> MSADSSPLVGSTPTGYGTLTIGTSIDPLSSSVSSVRLSGYCGSPWRVIGYHVVVWMMAGIPLLLFRWKPLWGVRLRLRPCNLAHAETLVIEIRDKEDSSWQLFTVQVQTEAIGEGSLEPSPQSQAEDGRSQAAVGAVPEGAWKDTALHKSEEAVSVGQKRVLRYYLFQGQRYIWIETQQAFYQVSLLDHGRSCDDVHRSRHGLSLQDQMVRKAIYGPNVISIPVKSYPQLLVDEALNPYYGFQAFSIALWLADHYYWYALCIFLISSISICLSLYKTRKQSQTLRDMVKLSMRVCVCRPGGEEEWVDSSELVPGDCLVLPQEGGLMPCDAALVAGECMVNESSLTGESIPVLKTALPEGLGPYCAETHRRHTLFCGTLILQARAYVGPHVLAVVTRTGFCTAKGGLVSSILHPRPINFKFYKHSMKFVAALSVLALLGTIYSIFILYRNRVPLNEIVIRALDLVTVVVPPALPAAMTVCTLYAQSRLRRQGIFCIHPLRINLGGKLQLVCFDKTGTLTEDGLDVMGVVPLKGQAFLPLVPEPRRLPVGPLLRALATCHALSRLQDTPVGDPMDLKMVESTGPQLQAMEEPPVPVSVLHRFPFSSALQRMSVVVAWPGATQPEAYVKGSPELVAGLCNPETVPTDFAQMLQSYTAAGYRVVALASKPLPTVPSLEAAQQLTRDTVEGDLSLLGLLVMRNLLKPQTTPVIQALRRTRIRAVMVTGDNLQTAVTVARGCGMVAPQEHLIIVHATGQPASLEFLPMESPTAVNGVKDPDQAASYTVEPDPRSRHLALSGPTFGIIVKHFPKLLPKVLVQGTVFARMAPE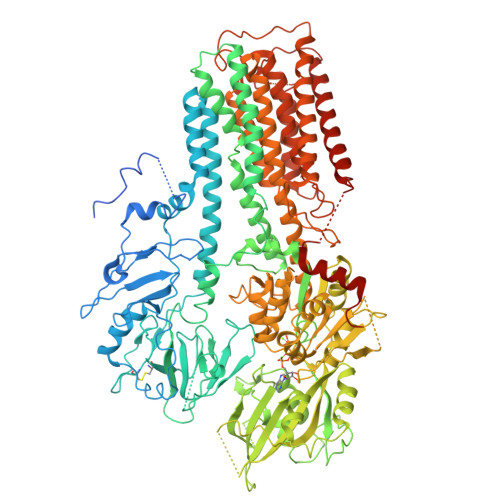QKTELVCELQKLQYCVGMCGDGANDCGALKAADVGISLSQAEASVVSPFTSSMASIECVPMVIREGRCSLDTSFSVFKYMALYSLTQFISVLILYTINTNLGDLQFLAIDLVITTTVAVLMSRTGPALVLGRVRPPGALLSVPVLSSLLLQMVLVTGVQLGGYFLTLAQPWFVPLNRTVAAPDNLPNYENTVVFSLSSFQYLILAAAVSKGAPFRRPLYTNVPFLVALALLSSVLVGLVLVPGLLQGPLALRNITDTGFKLLLLGLVTLNFVGAFMLESVLDQCLPACLRRLRPKRASKKRFKQLERELAEQPWPPLPAGPLR>MKIAIPKERRPGEDRVAISPEVVKKLVGLGFEVIVEQGAGVGASITDDALTAAGATIASTAAQALSQADVVWKVQRPMTAEEGTDEVALIKEGAVLMCHLGALTNRPVVEALTKRKITAYAMELMPRISRAQSMDILSSQSNLAGYRAVIDGAYEFARAFPMMMTAAGTVPPARVLVFGVGVAGLQAIATAKRLGAVVMATDVRAATKEQVESLGGKFITVDDEAMKTAETAGGYAKEMGEEFRKKQAEAVLKELVKTDIAITTALIPGKPAPVLITEEMVTKM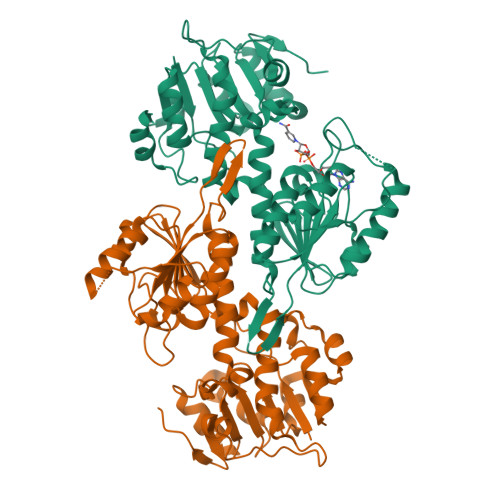KPGSVIIDLAVEAGGNCPLSEPGKIVVKHGVKIVGHTNVPSRVAADASPLFAKNLLNFLTPHVDKDTKTLVMKLEDETVSGTCVTRDGAIVHPALTGQGA[4x]> GSHMSQHGNRTFSYTLEDHTKQAFGIMNELRLSQQLCDVTLQVKYQDAPAAQFMAHKVVLASSSPVFKAMFTNG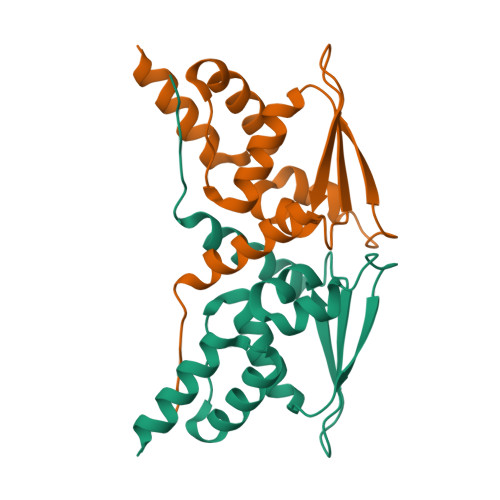LREQGMEVVSIEGIHPKVMERLIEFAYTASISMGEKCVLHVMNGAVMYQIDSVVRACADFLVQQLD> XK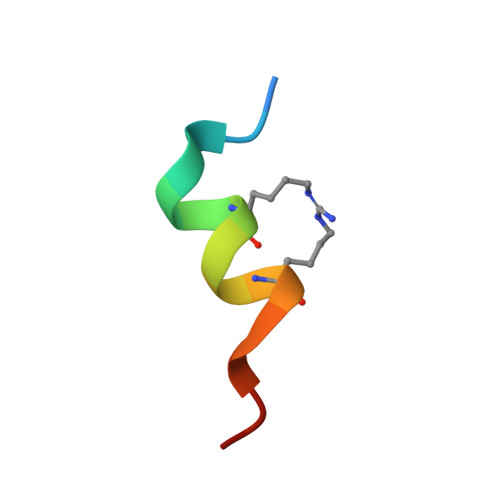ETAAALFERQHMDSX> SGSPSYTENKPDKKKKYMINDAKTIQLVGPLISSPDNLGFQKRSHKARELPRFLINQEPQLEKRAFVQDPWDKANQEKMISLEESIDDLNELYETLKKMRNTERSIMEEKGLVDKADSAKDLYDAIVFQGTCLDMCPTFERSRRNVEYTVYSYEKNQPNDKKASRTKALKVFARPAAAAAPPLPSDVRPPHILVKTLDYIVDNLLTTLPESEGFLWDRMRSIRQDFTYQNYSGPEAVDCNERIVRIHLLILHIMVKSNVEFSLQQELEQLHKSLITLSEIYDDVRSSGGTCPNEAEFRAYALLSKIRDPQYDENIQRLPKHIFQDKLVQMALCFRRVISNSAYTERGFVKTENCLNFYARFFQLMQSPSLPLLMGFFLQMHLTDIRFYALRALSHTLNKKHKPIPFIYLENMLLFNNRQEIIEFCNYYSIEIINGDAADLKTLQHYSHKLSETQPLKKTYLTCLERRLQKTTYKGLINGGED;> MDMANQLLDELAHGNFSHLTLNLSQNGREIAILQKQLTGFDDKQLETFVEQHPAMPNDTRFKIMCTSFLNYARDVDPWSAWSSSDLIFEFYQCLINCLINDNAPHIEMLIPVATRETEFIINLAGKLDSFHLQLHTRSHQFLSHISSILSRLFNSIKPPRGNASSTNIPGKQRILLYLVNKLNNIYFRIESPQLCSNIFKNFQPKSMLAHFNEY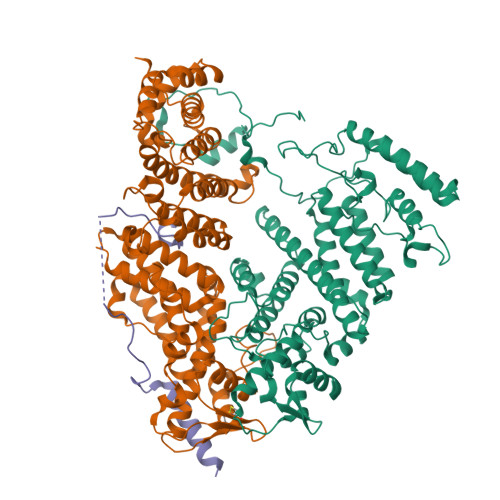QLDQQIEYRYLLGRYYLLNSQVHNAFVQFNEAFQSLLNLPLTNQAITRNGTRILNYMIPTGLILGKMVKWGPLRPFLSQETIDNWSVLYKHVRYGNIQGVSLWLRQNERHLCARQLLIVLLEKLPMVTYRNLIKTVIKSWTTEWGQNKLPYSLIERVLQLSIGPTFEDPGAQEITIYNGIHSPKNVENVLVTLINLGLLRANCFPQLQLCVVKKTTMIQEIVPPVNERITKMFPAHSHVLW;> MSTDVAAAQAQSKIDLTKKKNEEINKKSLEEDDEFEDFPIDTWANGETIKSNAVTQTNIWEENWDDVEVDDDFTNELKAELDRYKRENQ> MAGPIIAGKSESSELPRVEDRATFIYIEHAKINRVDSAVTVAEAKGVVRIPAAMIGVLLLGPGTDISHRAVELLGDTGTALVWVGEQGVRYYASGRALARSTRFLVKQAELVTNERSRLRVARRMYQMRFPTEDVSKLTMQQLRSHEGARVRRKYRELSKKYNV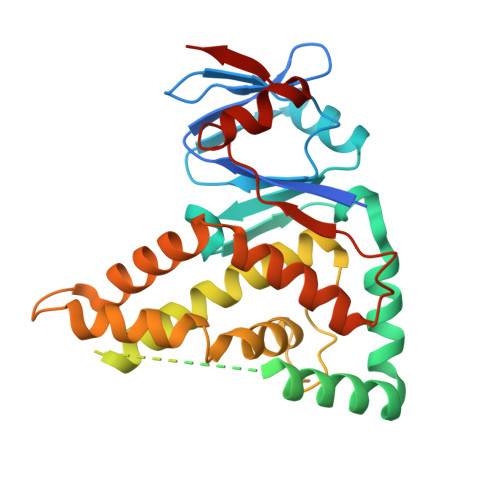PWKKRVYNPDDFAGGDPINQALSAAHVALYGLVHSVVAALGLSPGLGFVHTGHDRSFIYDVADLYKAEITVPIAFAVAAEAEEGQDIGQLARLRTRDAFVDGKILKRMVKDLQTLLEIPEEGQIEAEPLSLWDDKEKLVPYGVNYSEVTSCP>MQSSVNEFLTPRHIDVQVVSQTRAKITLEPLERGFGHTLGNALRRILLSSMPGCAVVEAEIDGVLHEYSAIEGVQEDVIEILLNLKGLAIKLHGRDEVTLTLAKKGSGVVTAADIQLDHDVEIINGDHVIANLADNGALNMKLKVARGRGYEPADARQSDEDESRSIGRLQLDASFSPVRRVSYVVENARVEQRTNLDKLVLDLETNGTLDPEEAIRRAATILQQQLAAFVDLKGDSEPVVEEQEDEIDPILLRPVDDLELTVRSANCLKAENIYYIGDLIQRTEVELLKTPNLGKKSLTEIKDVLASRGLSLGMRLDNWPPASLKKDDKATA[2x];> MAYSYTEKKRIRKDFSKLPDVMDVPYLLAIQLDSYREFLQAGATKEQFRDVGLHAAFKSVFPIISYSGNAALEYVGYRLGEPAFDVKECVLRGVTFAVPLRVKVRLIIFDRESSNKAIKDIKEQEVYMGEIPLMTENGTFIINGTERVIVSQLHRSPGVFFDHDRGKTHSSGKLLYSARIIPYRGSWLDFEFDPKDCVFVRIDRRRKLPASVLLRALGYSTEEILNAFYATNVFHIKGETLNLELVPQRLRGEVASIDIKDGSGKVIVEQGRRITARHINQLEKAGVSQLEVPFDYLIGRTIAKAIVHPATGEIIAECNTELTLDLLAKVAKAQVVRIETLYTNDIDCGPFISDTLKIDNTSNQLEALVEIYRMMRPGEPPTKEAAETLFGNLFFSAERYDLSAVGRMKFNRRIGRTEIEGPGVLSKEDIIDVLKTLVDIRNGKGIVDDIDHLGNRRVRCVGEMAENQFRVGLVRVERAVKERLSMAESEGLMPQDLINAKPVAAAIKEFFGSSQLSQFMDQNNPLSEITHKRRVSALGPGGLTRERAGFEVRDVHPTHYGRVCPIETPEGPNIGLINSLATYARTNKYGFLESPYRVVKDSLVTDEIVFLSAIEEADHVIAQASATLNEKGQLVDELVAVRHLNEFTVKAPEDVTLMDVSPKQVVSVAASLIPFLEHDDANRALMGSNMQRQAVPTLRADKPLVGTGMERNVARDSGVCVVARRGGVIDSVDASRVVVRVADDEVETGEAGVDIYNLTKYTRSNQNTCINQRPLVSKGDVVARGDILADGPSTDMGELALGQNMRVAFMPWNGFNFEDSICLSERVVQEDRFTTIHIQELTCVARDTKLGPEEITADIPNVGEAALNKLDEAGIVYVGAEVQAGDILVGKVTPKGETQLTPEEKLLRAIFGEKASDVKDTSLRVPTGTKGTVIDVQVFTRDGVERDSRALSIEKMQLDQIRKDLNEEFRIVEGATFERLRAALVGAKAEGGPALKKGTEITDDYLDGLERGQWFKLRMADDALNEQLEKAQAYISDRRQLLDDKFEDKKRKLQQGDDLAPGVLKIVKVYLAIKRRIQPGDKMAGRHGNKGVVSVIMPVEDMPHDANGTPVDIVLNPLGVPSRMNVGQILETHLGLAAKGLGEKINRMLEEQRKVAELRKFLHEIYNEIGGREENLDELGDNEILALAKNLRGGVPMATPVFDGAKEREIKAMLKLADLPESGQMRLFDGRTGNQFERPTTVGYMYMLKLNHLVDDKMHARSTGSYSLVTQQPLGGKAQFGGQRFGEMEVWALEAYGAAYTLQEMLTVKSDDVNGRTKMYKNIVDGDHRMEAGMPESFNVLIKEIRSLGIDIELETE;> MKDLLNLLKNQGQIEEFDAIRIGLASPEMIRSWSFGEVKKPETINYRTFKPERDGLFCAKIFGPVKDYECLCGKYKRLKHRGVICEKCGVEVALAKVRRERMGHIELASPVAHIWFLKSLPSRIGLLLDMTLRDIERVLYFESYVVIDPGMTTLEKGQLLNDEQYFEALEEFGDDFDARMGAEAVHELLNAIDLEHEIGRLREEIPQTNSETKIKKLSKRLKLMEAFQGSGNKPEWMVLTVLPVLPPDLRPLVPLDGGRFATSDLNDLYRRVINRNNRLKRLLDLAAPDIIVRNEKRMLQEAVDALLDNGRRGRAITGSNKRPLKSLADMIKGKQGRFRQNLLGKRVDYSGRSVITVGPTLRLHQCGLPKKMALELFKPFIFGKLEGRGMATTIKAAKKMVERELPEVWDVLAEVIREHPVLLNRAPTLHRLGIQAFEPVLIEGKAIQLHPLVCAAYNADFDGDQMAVHVPLTLEAQLEARALMMSTNNILSPANGEPIIVPSQDVVMGLYYMTREAINAKGEGMAFADLQEVDRAYRSGQASLHARVKVRINEKIKGEDGQLTANTRIVDTTVGRALLFQVVPAGLPFDVVNQSMKKKAISKLINHCYRVVGLKDTVIFADQLMYTGFAYSTISGVSIGVNDFVIPDEKARIINAATDEVKEIESQYASGLVTQGEKYNKVIDLWSKANDEVSKAMMANLSKEKVVDREGKEVDQESFNSMYMMADSGARGSAAQIRQLAGMRGLMAKPDGSIIETPITANFREGLNVLQYFISTHGARKGLADTALKTANSGYLTRRLVDVAQDLVVTEIDCGTEHGLLMSPHIEGGDVVEPLGERVLGRVIARDVFKPGSDEVIVPAGTLIDEKWVDFLEVMSVDEVVVRSPITCETRHGICAMCYGRDLARGHRVNIGEAVGVIAAQSIGEPGTQLTMRTFHIGGAASRTSAADNVQVKNGGTIRLHNLKHVVRADGALVAVSRSGELAVADDFGRERERYKLPYGAVISVKEGDKVDPGAIVAKWDPHTHPIVTEVDGTVAFVGMEEGITVKRQTDELTGLTNIEVMDPKDRPAAGKDIRPAVKLIDAAGKDLLLPGTDVPAQYFLPANALVNLTDGAKVSIGDVVARIPQETSKTRDITGGLPRVADLFEARRPKEPSILAEISGTISFGKETKGKRRLVITPNDGSDPYEELIPKWRHLNVFEGEQVNRGEVISDGPSNPHDILRLLGVSSLAKYIVNEIQDVYRLQGVKINDKHIETILRQMLRKVEVSESGDSSFIKGDQVELTQVLEENEQLGTEDKFPAKYERVLLGITKASLSTESFISAASFQETTRVLTEAAVTGKRDFLRGLKENVVVGRLIPAGTGLAYHSERKRQRDLGKPQRVSASEAEAALTEALNSSGN;> MARVTVEDCLDNVDNRFELVMLATKRARQLATGGKEPKVAWENDKPTVVALREIASGLVDENVVQQEDIVEDEPLFAAFDDEANTEAL;> MFQSTEQALAVAYWMFEQQPGPRSSTAMVIDSLRERFDRRFIERLPSGLSPHEWQAQAVMTVRFAQRQLAAHPLELAVVRAEFARGRDFVLGLAALRDWLKPAAGPIEQRAALALLMRMFRRPPSSIREIERLSGLSKSTLHRWDKEWRERVAALLRQALLRLEEPMAQVGIVCEH

AlpA positively regulates a programmed cell death pathway linked to the virulence of Pseudomonas aeruginosa by recognizing an AlpA binding element within the promoter, then binding RNA polymerase directly and allowing it to bypass an intrinsic terminator positioned downstream. AlpA then positively regulates the cell lysis genes alpBCDE by functioning as a processive antiterminator. In particular, AlpA recognizes a putative AlpA binding element (ABE) located between the −10 and −35 elements of the alpB promoter (PalpB), binds RNAP directly, and allows it to bypass an intrinsic termination site (tB) positioned downstream of PalpB. Like 21Q, AlpA forms a narrow ring inside the RNA exit channel and renders RNAP resistant to termination signals by prohibiting RNA hairpin formation.

To prepare an AlpA-loaded complex, we performed in vitro transcription with a DNA template comprising promoter PalpB, followed by a 68-bp C-less cassette containing a consensus −10-like sequence, followed by a CC-halt site, using Pae RNAP-σ70 holoenzyme, AlpA, and GreB, in the presence of an NTP subset lacking CTP. The structure of the AlpA-loaded complex was determined at a nominal resolution of 3.7 Å. Extensive 3D classification did not reveal a complex with both AlpA and σ70, indicating that σ70 is released upon the formation of a loaded complex. The structure of the AlpA-loaded complex reveals AlpA interacting with the RNA exit channel and having the RNA 5′ end threaded into and through its ring. The conformation and interactions of AlpA in the loaded complex are similar to those in the loading complex. Notable changes include a rotation of the AlpA C-terminal segment as a rigid body associated with the loss of AlpA-DNA interactions in the loaded complex, and a disorder-to-order transition in L1 associated with the gain of AlpA-RNA interactions in the loaded complex. Clear, traceable density is present for the 14 nucleotides (nt) at the 3′ end of the RNA product: 2 nt of RNA are located upstream of the AlpA ring, outside the RNA exit channel; 3 nt of RNA are located downstream of the AlpA ring, in the RNA exit channel; and 9 nt of RNA are base paired with the template strand DNA as an RNA–DNA hybrid. According to the structure of the AlpA-loaded complex, the ring-like structure of AlpA inserts into the RNA exit channel and serves as a molecular nozzle. The inner diameter of the nozzle is <14 Å (the shortest distance between Cαs), which is too small to accommodate an RNA hairpin (diameter > 20 Å). Therefore, we infer that AlpA renders RNAP resistant to intrinsic termination by prohibition RNA hairpin formation in the RNA exit channel.> DNLRHFVQDYAVRALIPYIEHLVAILAEGVTNKKGVSKSLLSATKRWFVTSKPGAGANNQNAVIYTNESAELQTRKLGDLYFMFGHYNLAFQSYHQAKR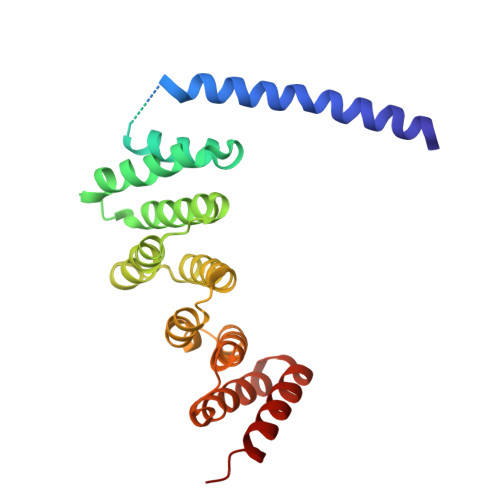DFNADSAWQYYAGALEMAALSAFMLGTAQRKTYDYMEDAIVCYLTVCKLQQFATRATLLSMECLKTARLYSEVAKQLIRMTNEESDLRSALLLEQAAYCFLVTQPPMHRKYAFHIVLAGNRYSRAGQRKHAYRCYRQAYQVFQKREW> FTLIELMIVIAIVGILAAVALPAYQD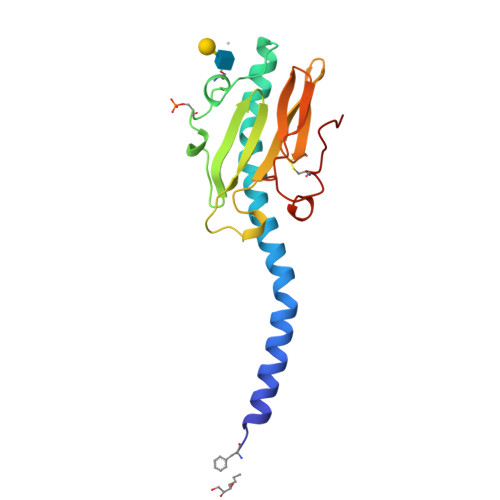YTARAQVSEAILLAEGQKSAVTEYYLNHGKWPENNTSAGVASPPSDIKGKYVKEVEVKNGVVTATMLSSGVNNEIKGKKLSLWARRENGSVKWFCGQPVTRTDDDTVADAKDGKEIDTKHLPSTCRDNFDAK> EPVEEEDPFFKVPVNKLAAAVSNFGYDLYRLRSSASPTGNVLLSPLSVATALSALSLGAEHRTESVIHRALYYDLITNPDIHSTYKELLASVTAPEKNLKSASRIVFERKLRVKSSFVAPLEKSYGTRPRILTGNPRVDLQEINNWVQAQMKGKIARSTREMPSALSILLLGVAYFKGQWVTKFDSRKTTLQDFHLDEDRTVRVPMMSDPKAILRYGLDSDLNCKIAQ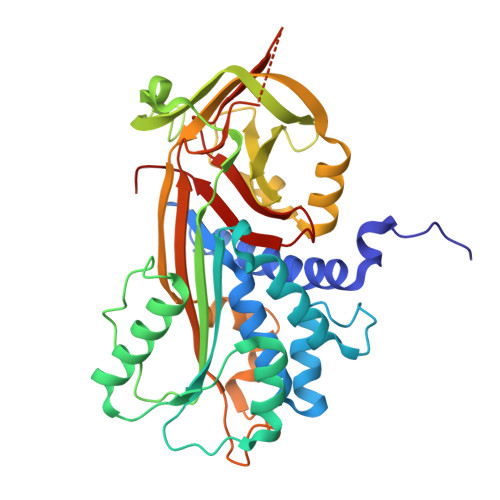LPLTGSMSIIFFLPLTVTQNLTMIEESLTSEFIHDIDRELKTIQAVLTVPKLKLSFEGELTKSLQDMKLQSLFESPDFSKITGKPVKLTQVEHRAAFEWNEEGAGSSPSGLQVRTFPLDYHLNQPFLFVLRDTDTGALLFIGRILDPSS>[2x]SNAMAAFKDHFTPVADAYRAFRPRYPRALFRWLGEVAPARGDALDCGCGSGQASLGLAEFFERVHAVDPGEAQIRQALRHPRVTYAVAPAEDTGLPPASVDVAIAAQAMHWFDLDRFWAELRRVARPGAVFAAVTYGLTRVDPEVDAVVDRLYHGLLARDWPP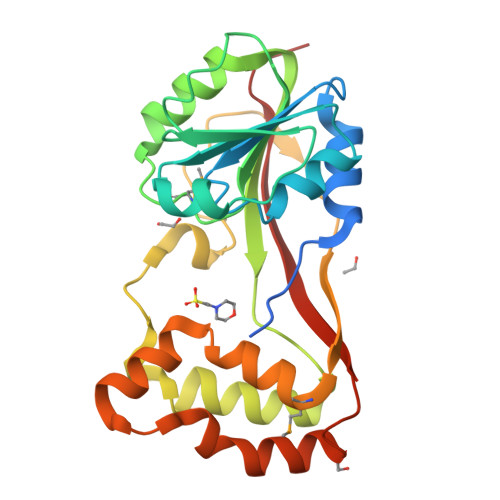ERVHVESGYRTLPFPFPELEAPPLEIEERWPMDAFLGYLGTWSAVTAHRRRTGADPLAEIAPALRAAWGTPERPLRVTWPIAIRAGRILPHAGG2-methyl-N-(2-{[2-(trifluoromethyl)phenyl]sulfanyl}ethyl)-2-[5-(trifluoromethyl)pyridine-2-sulfonyl]propanamide 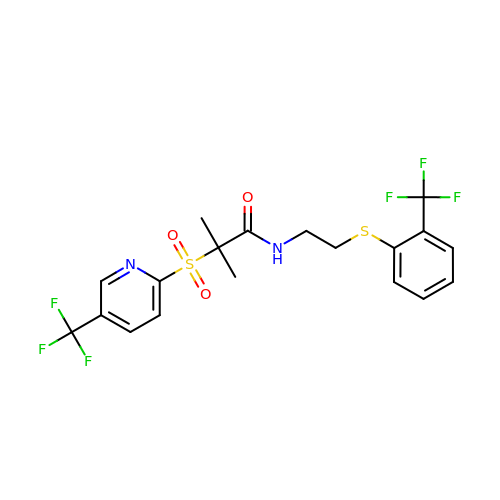| C19 H18 F6 N2 O3 S2 | LUNHBUGYRUFQHM-UHFFFAOYSA-N> MHREVILCKDQDGKIGLRLKSIDNGIFVQLVQA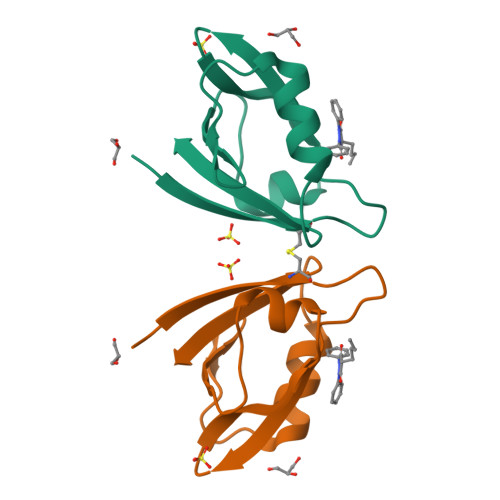NSPASLVGLRFGDQVLQINGENCAGWSSDKAHKVLKQAFGEKITMTIR>SLFELGKMILQETGKNPAKSYGAYGCNCGVLGRGGPKDATDRCCYVHKCCYKKITGCDPKKDRYSYSWKDKTIVCGENNPCLKELCECDKAVAICLRENLGTYNKKYRY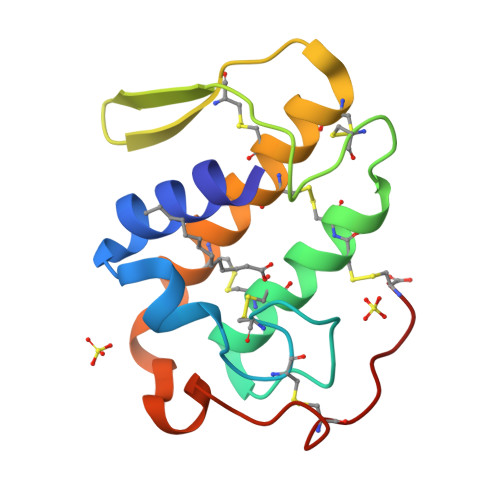HLKPFCKKADPC[2x]>[2x]MKTPRRRMRLAVFKALFQHEFRRDEDL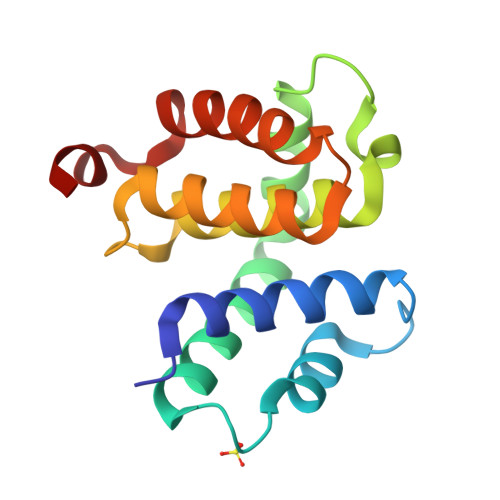EQILEEILDETYDKKAKEDARRYIRGIKENLSMIDDLISRYLEKWSLNRLSVVDRNVLRLATYELLFEKDIPIEVTIDEAIEIAKRYGTENSGKFVNGILDRIAKEHAPKEKFEL3-methyl-4-(3-methyl-4-oxidanylidene-5,6,7,8-tetrahydro-2~{H}-cyclohepta[c]pyrrol-1-yl)benzamide 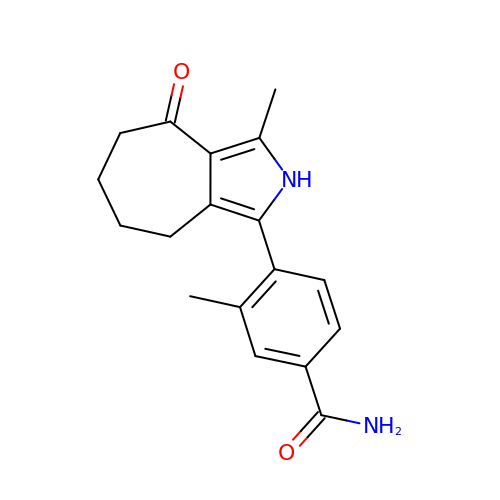| C18 H20 N2 O2 | ATVBLDDCYXMXQS-UHFFFAOYSA-N(3aR,8S,9aS)-2-[(trifluoromethyl)sulfonyl]decahydro-3a,8-epoxypyrrolo[3,4-c]azocine | C10 H15 F3 N2 O3 S | 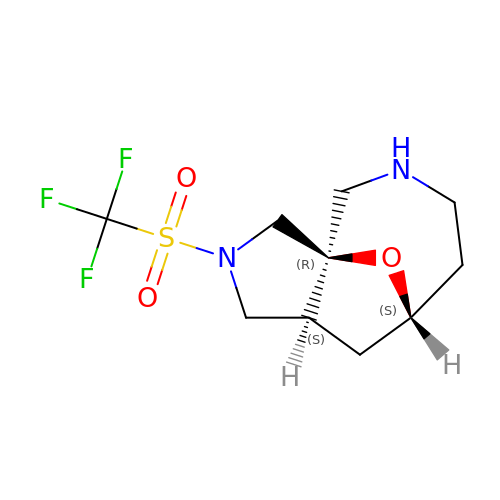SDCYRSFOCAJCPQ-DJLDLDEBSA-N>MDSSTATAMTAPFIDPTDHVNLKTDTDASENRRMGNYKPSIWNYDFLQSLATHHNIVEERHLKLAEKLKGQVKFMFGAPMEPLAKLELVDVVQRLGLNHLFETE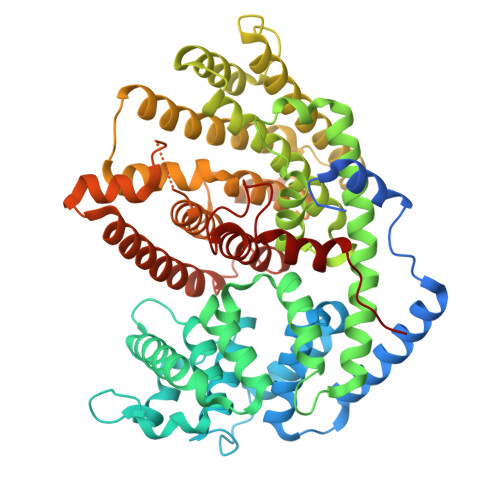IKEALFSIYKDGSNGWWFGHLHATSLRFRLLRQCGLFIPQDVFKTFQNKTGEFDMKLCDNVKGLLSLYEASYLGWKGENILDEAKAFTTKCLKSAWENISEKWLAKRVKHALALPLHWRVPRIEARWFIEAYEQEANMNPTLLKLAKLDFNMVQSIHQKEIGELARWWVTTGLDKLAFARNNLLQSYMWSCAIASDPKFKLARETIVEIGSVLTVVDDGYDVYGSIDELDLYTSSVERWSCVEIDKLPNTLKLIFMSMFNKTNEVGLRVQHERGYNSIPTFIKAWVEQCKSYQKEARWFHGGHTPPLEEYSLNGLVSIGFPLLLITGYVAIAENEAALDKVHPLPDLLHYSSLLSRLINDIGTSPDEMARGDNLKSIHCYMNETGASEEVAREHIKGVIEENWKILNQCCFDQSQFQEPFITFNLNSVRGSHFFYEFGDGFGVTDSWTKVDMKSVLIDPIPLGEE[4x]>[2x]MADYKDDDDKGTDYKDDDDKLEVLFQGPMEANQCPLVVEPSYPDLVINVGEVTLGEENRKKLQKIQRDQEKERVMRAACALLNSGGGVIRMAKKVEHPVEMGLDLEQSLRELIQSSDLQAFFETKQQGRCFYIFVKSWSSGPFPEDRSVKPRLCSLSSSLYRRSETSVRSMDSREAFCFLKTKRKPKILEEGPFHKIHKGVYQELPNSDPADPNSDPADLIFQKDYLEYGEILPFPASQLVEFKQFSTKHFQEYVKRTIPEYVPAFANTGGGYLFIGVDDKSREVLGCAKENVDPDSLRRKIEQAIYKLPCVHFCQPQRPITFTLKIVNVLKRGEL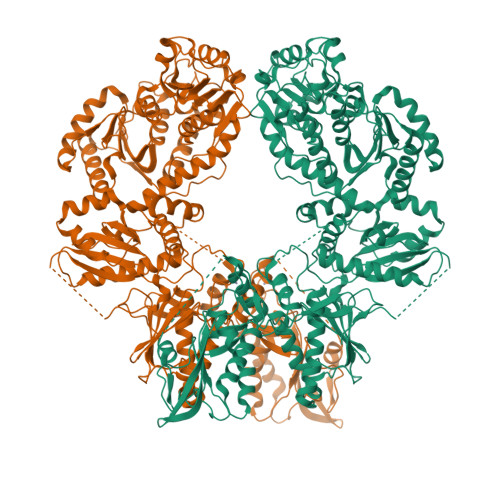YGYACMIRVNPFCCAVFSEAPNSWIVEDKYVCSLTTEKWVGMMTDTDPDLLQLSEDFECQLSLSSGPPLSRPVYSKKGLEHKKELQQLLFSVPPGYLRYTPESLWRDLISEHRGLEELINKQMQPFFRGILIFSRSWAVDLNLQEKPGVICDALLIAQNSTPILYTILREQDAEGQDYCTRTAFTLKQKLVNMGGYTGKVCVRAKVLCLSPESSAEALEAAVSPMDYPASYSLAGTQHMEALLQSLVIVLLGFRSLLSDQLGCEVLNLLTAQQYEIFSRSLRKNRELFVHGLPGSGKTIMAMKIMEKIRNVFHCEAHRILYVCENQPLRNFISDRNICRAETRKTFLRENFEHIQHIVIDEAQNFRTEDGDWYGKAKSITRRAKGGPGILWIFLDYFQTSHLDCSGLPPLSDQYPREELTRIVRNADPIAKYLQKEMQVIRSNPSFNIPTGCLEVFPEAEWSQGVQGTLRIKKYLTVEQIMTCVADTCRRFFDRGYSPKDVAVLVSTAKEVEHYKYELLKAMRKKRVVQLSDACDMLGDHIVLDSVRRFSGLERSIVFGIHPRTADPAILPNVLICLASRAKQHLYIFPWGGH>SHGNIDLGFIYTMGAHTVPELVQNFTKVESHKDITFSFFQGATKSIIPDLKNEKFDLAICSYVENEPDIEFLPLTKQELVVVVAENHPLAKYDSIDLQDTADYSYIFFSDTSGLRPLIDSLFAEINIQPKIGCYVEEDTAMVGLVSVDYGISIM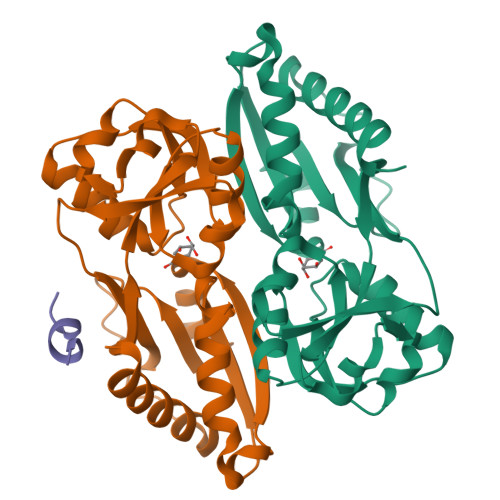PKISSLAHYNVKVLSINEPKHDRFIYLASLKNHYISPASKAFKDFALRYGKKHFLRENLYFQGLEHHHHHHH[2x];> GAYGAGLAH> GHHHHHHMQAALL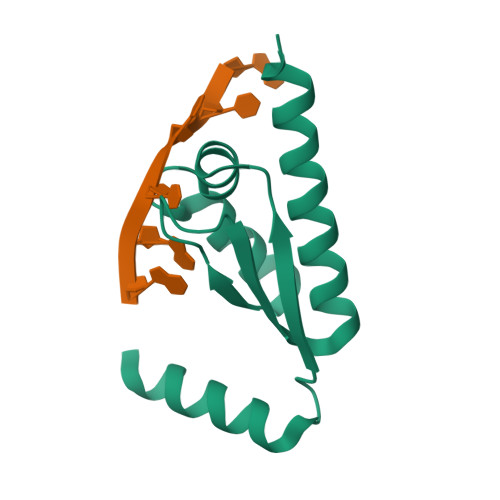RRKSVNTTECVPVPSSEHVAEIVGRQGCKIKALRAKTNTYIKTPVRGEEPIFVVTGRKEDVAMAKREILSAAEHFSMIRAS> MSVRDEFDAWAADGRDKGMEDRHWHTAKHALARM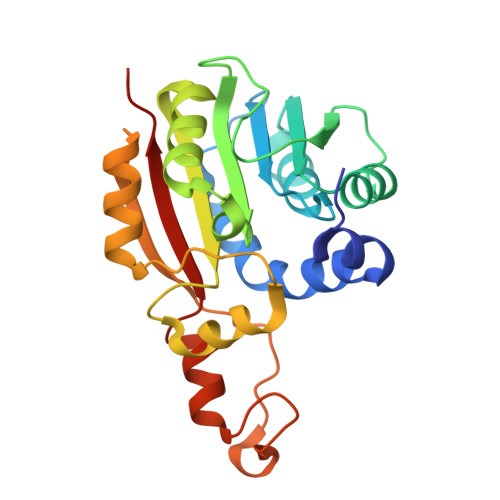PVEEGDTVVDLGTGSGYALRALRDTKGIGRGFGLDGSPEMVQNARAYTDTDDLSFLVGDFDDLPFDDDSVDHVWSMEAFYYAADPHHTLEEIARILKPGGTFYCAVNYYEENVHSHEWQEHISIDMTRWSHAEYREAFRDAGLHVAEQDSIADLDIDIPAATEFPTDDWETREAMVERYRTFGTLLTVGVAPHHHHH> MFGLIGHLTSLEQARDVSRRMGYDEYADQGLEFWSSAPPQIVDEITVTSATGKVIHGRYIESCFLPEMLAARRFKTATRKVLNAMSHAQKHGIDISALGGFTSIIFENFDLASLRQVRDTTLEFERFTTGNTHTAYVICRQVEAAAKTLGIDITQATVAVVGATGDIGSAVCRWLDLKLGVGDLILTARNQERLDNLQAELGRGKILPLEAALPEADFIVWVASMPQGVVIDPATLKQPCVLIDGGYPKNLGSKVQGEGIYVLNGGVVEHCFDIDWQIMSAAEMARPERQMFACFAEA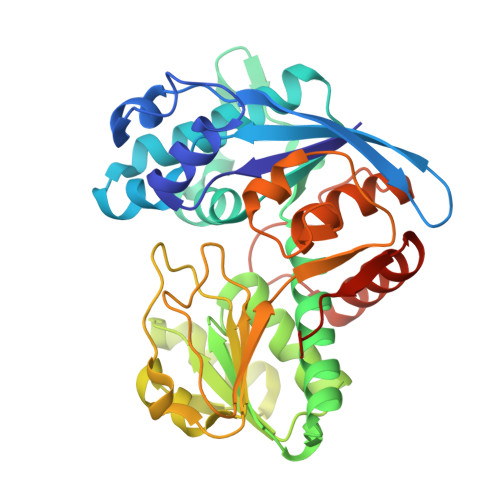MLLEFEGWHTNFSWGRNQITIEKMEAIGEASVRHGFQPLALAIENLYFQ> MATQKETTRKRDKSVNFRLGLRNMLAQIHPDISVQTEALSELSNIAVFLG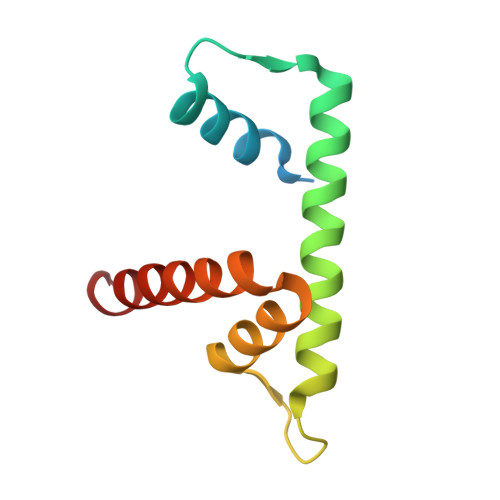KKISHGAVTLLPEGTKTIKSSAVLLAAGDLYGKDLGRHAVGEMTKAVTRYGSAK>[2x]ARPAFVNKLWSMVNDKSNEKFI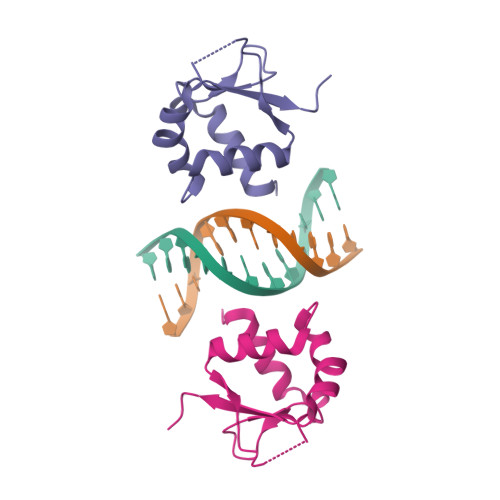HWSTSGESIVVPNRERFVQEVLPKYFKHSNFASFVRQLNMYGWHKVQDVKSGSMLSNNDSRWEFENERHA> RRNVEARGIRRSPVVTPDIQIGHGEDAIEMDLYRYLLSNRIIFIGGYINDKMATQIVGSLMALEAVDENEDIRIYINSPGGQPYSVLGVVDAMQSIKPDVQTVALGACYSYASLVVAAGTKGKRYAMKNTRLMMTQPMGGSQGDIYQIKATVEELNALYQIFSRYYMKFTGMNQDQIEQATCRDHFMTPEQAKLEGLIDEIIRGKGDYTVPPAIVRQFREVGLVDDLTPGPFLKVDCN;>ARRSVAARSSAPELWTPTSEVKLAVSSRNPHPPVVCQGPPPPNPLVIERFQGVVSQLFQQRIVRLGGAVDDDMANLLVAQLLYLDSVDNKRDITMYVNSPGGSVTAGMAVFDTMRHIRPDVSTCCIGLAASMGAFILASGQAGKRYSLPNSRIMIHQPLGGAQGQATDIEIQANEILHHKLTLNGYLAQFTGQSMETITKDTDRDFFMSPQEAIEYGLVDAIISKPQMLQSREVALSS[3x];>NSQPIVAPRTAEMQGDPFGLLLRQRIVFLGGEVEDFGADAIISQLLLLDSQDPTKDIKIFINSPGGSVTAGMGIYDAMMLCRADVNTYCFGLAASMGAFLLGAGKRGKRNSMPNSRIMIHQPLGGASGQAVDIEIQAKEIMYHKANLNRIMADYCQQPLSKIEEDTDRDRYMSPLEAKEYGLIDHIIGGEEAVFNVKGSLKKFPKIKEEFVTDKDDMVKRNIMDGDPFLSETPSWRFKSPQTEPYMPSQAPGSRWFRTRKVSKEDYKEMQEQRQAELMAESDDGKKSVKDRIDDAW[3x];>[3x]NYLDQGALNNESGRSLYRKQTERVIQEEESKKVFMIINSFGGSVGNGITVHDALQFIKAGSLTLALGVAASAASLALAGGTIGERYVTEGCHTMIHQPEGGLNGQASDIWIDSQEIMKIRLDVAEIYSLSTYRPRHKILRDLDRDFYLTAMETIYYGLADEIATNEVMHSIVEMTNQVWSYHDSKQERLLESRASLVGDSTQTQESNS;> AYGDYPNYPEGRPLFLPEAERFGNPPDLPSLLLQQRVIYISMPFLPSVTELVVAQCYYLDFDDRNRQRPIYVYLNSTGCINDKGQAISADNEFYAIWAALGFTRAPLYTGVTWKAQNQAAVLLSAGQKGHRYSFPHAKISTAPPVMNRVFGQAVDAQLQANELDYATKYYAAILARSTGKDLETCQKQYLSRKRYFSVKEAYEEGLVDKLVPGFMLNRFRKMQKDAGVGEEDLFDMNKPKFKFRRQ;> RKLSHLRKKLWKEAGPPPDLATRLFSERIMYLGMPIDSSVAELLTAQLFVLVQEAPDPIFFYINSTGIAKSTTKFGNEHEAIAVYSMMKGVQKYCPIYTLCVGNAFGEAALLLSAGSPGKRAALRSSTIMLRQPLQRLGGMQASDIDIYRKITREKTATMAKYLAACTKKTEEQIMTDFTRPRYFNPYEAVSYGLIDTVLEPKEERAVFKDWEKMGSEIADLGLWDDEEQPLPTNIMYPGTSQYWRSDFDG;> KKSPQGFWQVTTKQISAAKRSGAPKRKVTTMMPVSVPKVLCRPPGQRQSEWVDLWEAYTYQKVVFIKEAITEDVANNMIALTLYLDSLDQKRIYYWLNVPGGDVVPTLALYDTMQYVRSKTATVCYGLCLGMGGFLLTAGGEKGYRFAMPHSILMMHHPSGASRGQASEMHIESRELVRMRDYLSLLTSNATGQPYDRVIRELSRNKWMDPKQAIEYGMIDKVLTTPMPKMPSTGPSFKFERQNDELIGL;> LVVHARASRYDRRKPPPPDLPSLLFDQRIVYLGMPLVPAVTELMVAELLYLEKQGATLPIEMLINSSGTTRQDGEILSFDSEGVALTSTMGFIKNPISTVNMGLAVGWSCVVLSFGRKGWRKSLPHSLAMIQQPRVPPTGQRQAIEVHIKWREVLDYKRELLRMFSLGTGLPVDKLDADMQRPLYMRPQDALEYGIIDEIIEPNEDKAEKAAQYWIRSGRAESEGRLEQWQEYLSLQEEYALKDSFRKVMTQDLRAAYRDTSSKLLKNSSRNMEQVQEFKERLPDDMLTENDEVRLPFSRDGVKLAILNAECYAERNIARQVAANKVSVPDKWRAAYAARPAPAAPAAEVDYDALIRAVEAMDEKAFATTDLDTLVEQYRVPA;> ATATAAPSELDDVGVSAAAESIIQYAINFARASETYEVHSWMVLMGILKYETCTAAKILKSLGLEDLYGAWNEVLWALNVCDGLQPRSFVTDIKFADRAFKVITAASDFAVWHGKDKMYSEDVLMALAAGGVLEDLFPDLNLSFERVRKAVEKESGRRYQLPDETEEAGPLKSEDDVSFL;> AASVTAEKAALDITKMTPIHDRVLIRPIEEEQKTAGGILLPKAPPKANSDAHIGEVLAVGSDVTLAVAKGDMVVFQKYAMAEVEVKEGQIIFVAEKSIMGKLE;> EAISVPAPFTKVAPKGDRVLVKVAEEEVKTRGGILLPPSAIKKPTSGEVVQLGDGRVGDGEVRPFYLQPGQTVVYSKFGFMYQDLKLSNGEEYILIREDDVIGIMPRANAQADDVPELQPLADRVLIKVEEVADVTMGGVFLPETAKERPLSGTVVRVGPGKYDKDAEGKRRTVPLAPGDKVLYFKYAGDNMETPSGDKFVVLRSDDVLCKA;>[2x]ATPVPKQFKAVKPVGDRVLVKVDKEEAKSVGGVLLPASVRNKPTAGSIIALGDAKSVKLS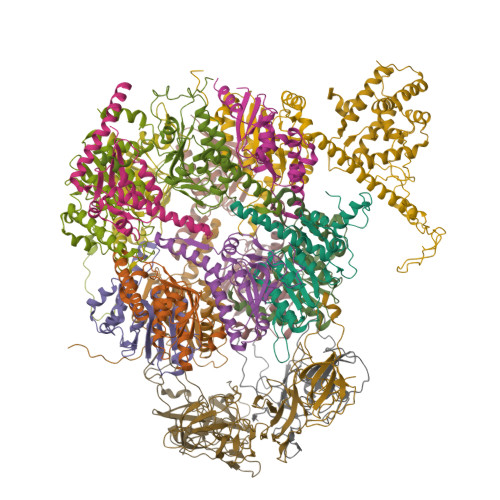DKVIYSKFAGTELELGGAEHVLLKEEDVIGVLSASEKIAQLKPLSDRILIKGAKAEDKTSGGVLLATESAEKPTFGTVVAVGEGREDEETKALVKPNVTVGATVMYSKYSGTEFEEDGDNYIVVRESDILAQLS> SNARNKIFISHAAPDDNDFTKWLALKLIALGYEVWCDVLFLDKGADFWKVIDKEIREGAIKFLLATSEIAIKRDGVLKEIAVAEKVKKQLKDDNFIIPLIIDENLSYDDLPPEIIRLNAVDFKKSWAVGLQDLLKALDDQKVEKNSPDPDKSNALYQQIFLHNKGIIEREEIYDSNWFSILSFPKELRFHDYEKLMPKGFDVRELTYPAVRYKNYLCTFAWEYDFMHQLPKTETYNSSQTIRIPTEEILSGKYDSPFIGNFECQRLIVQLLNKAFELRMKEKGVREYPMSNKMGYWFEKGKLEKDKFNKVLLVGKQKDKHWHFGISAAGKLYPFPVLMISSHIFFTKDGKELIESKKIQHAARRRQGKNWWNDDWRNKLLAFVKYLSDDENSFYLEVGSEEKIYISNEPVQFVGKVSYNMPEKNNLKDEAEISDLNDLNEFDGEIFEETDSE;> MKELIYIHEPNILFANGQKCADPRDGLALFGPFTKIYGIKSGVVGTQYGLSIFKNYINHIQKPIYNANNITRPMFPGFEAVFGCKWDADNVVFKEVTKEEIEKILYTESNHKRTYDLVSLFINKIITANKNEDEKVDVWFLVIPDEIYQYCR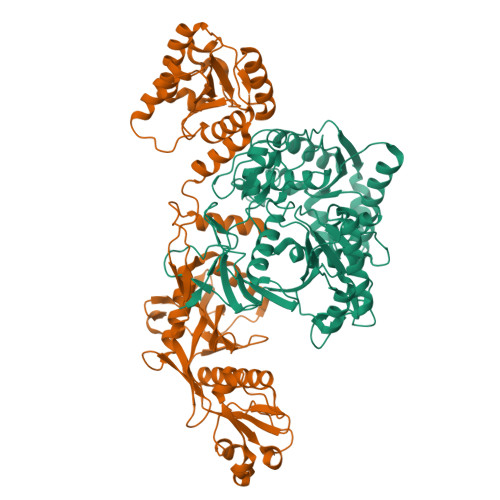PNSVLPKDLVQTKSLITKSKAKSFRYEPTLFENINKELKEQEKEAITYNYDAQFHDQLKARLLEHTIPTQILRESTLAWRDFKNKFGAPKRDFSKIEGHLAWTISTAAFYKAGGKPWKLSDIRSGVCYLGLVYKQIEKSSNPKNACCAAQMFLDNGDGTVFKGEVGPWYNQEKHEFHLNPKEAKALLTQALNSYKEQNGVFPKEIFIHAKTKFNGQEWNAFQEVTPEGTNLVGVTITKTKPLKLFKSEGNYPIMRGNAFIVNERSAFLWTVGYVPKTESTLSMEVPNPIFIEINKGEADIEQVLKDVLALTKLNYNACIYADGVPVTLRFADKIGEILTASTELKAPPLAFKYYI> MELIKGQALFLELDKKDFLSLKNNDKNIPTFAHPKNQEKILAIFSLPYKNPPQNTKLIAFYKDKKEEIFIKTLEGNYKSEKLQVENKKIFPPKTIQERIAKELKEANAIYSSYTPKALFNGAFNIPLNSFITSDFGKARTFNEKVASYHSGTDFRAATGTPIYAANSGVVKIAKDRYFAGNSVVIDHGFGIYSQYYHLSKIDVKVGQKIKKGELIGLSGASGRVSGPALHFGILAGGKQVDPLDFVSKFNAIFQL

We have described herein the reactions and the structure of Pgp3, a Csd protein of C. jejuni. This enzyme turns over the cell-wall peptidoglycan by both the d,d-endopeptidase and d,d-carboxypeptidase activities, as documented by mass spectrometric characterization of the requisite reactions with synthetic cell-wall fragments. The Pgp3 monomer is structurally divided into four regions: the N-terminal domain (NTD, residues 21–95), a flexible linker (residues 96–147), the LytM domain (residues 148–259), and the C-terminal helix (residues 260–273). The Pgp3 LytM domain contains a highly conserved tetrahedral Zn2+-ion-binding motif (H168xxxD172 and HxH249).

By using the H247A mutant variant, we successfully solved two structures of Pgp3 in complex with a pentapeptide (1, Ac-l-Ala1-γ-d-Glu2-mDAP3-d-Ala4−d-Ala5) and with a crosslinked muramyl tetra-tri peptide (2, NAM-l-Ala1-γ-d-Glu2-mDAP3-d-Ala4−mDAP3-γ-d-Glu2-l-Ala1-NAM). In the presence of the crosslinked heptapeptide (tetra-tri peptide), excellent electron density was seen for mDAP3-d-Ala4−mDAP3. The importance of these two complexes is that the scissile bond in the peptide substrate was seen bound within the active site. The tetra-tri peptide fragment (mDAP3-d-Ala4-mDAP3) mainly interacted with Pgp3 via its two terminal mDAP moieties. Tyr129, Arg195, and Tyr215 of Pgp3 contributed to the binding by forming several hydrogen-bonding networks. The hydroxyls of Tyr129 and Tyr215 were bound to O7 and O8 atoms of mDAP3 (from the donor strand) via hydrogen bonds (3.0 Å and 2.5 Å, respectively). The NH1 atom of Arg195 formed a salt bridge with mDAP3 (from the donor strand). The O5 and N1 atoms of the other mDAP3 moiety (from the acceptor strand) formed hydrogen bonds with the backbone nitrogen atoms of Val243 and Ser244. Importantly, the N1 and N4 atoms of the two mDAP of the tetra-tri peptide are responsible for linkage with the Glu2-Ala1-NAM moiety, which are solvent-exposed through the channels A and B, respectively. When we superimposed the structure of the H247A variant of Pgp3 in complex with the tetra-tri peptide with that of the WT complex with citrate (closed form), it was clear that the penta- or tetra-tri peptide cannot enter the active site in the closed conformation.>[3x]MEQTEKSKVYAENG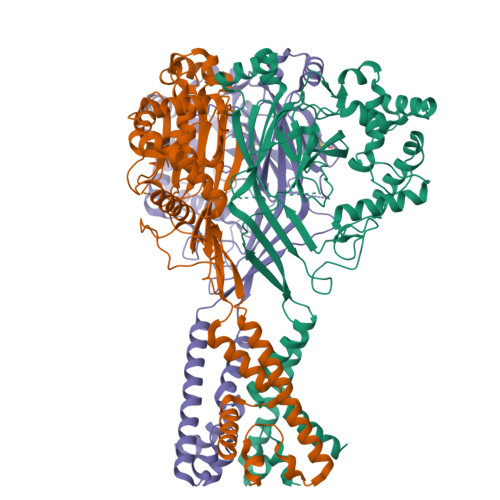LLEKIKLCLSKKPLPSPTERKKFDHDFAISTSFHGIHNIVQNRSKIRRVLWLVVVLGSVSLVTWQIYIRLLNYFTWPTTTSIEVQYVEKMEFPAVTFCNLNRFQTDAVAKFGVIFFLWHIVSKVLHLQEITANSTGSREATDFAASHQNFSIVEFIRNKGFYLNNSTLLDCEFFGKPCSPKDFAHVFTEYGNCFTFNHGETLQAKRKVSVSGRGLSLLFNVNQEAFTDNPALGFVDAGIIFVIHSPKKVPQFDGLGLLSPVGMHARVTIRQVKTVHQEYPWGECNPNIKLQNFSSYSTSGCLKECKAQHIKKQCGCVPFLLPGYGIECDLQKYFSCVSPVLDHIEFKDLCTVGTHNSSCPVSCEEIEYPATISYSSFPSQKALKYLSKKLNQSRKYIRENLVKIEINYSDLNYKITQQQKAVSVSELLADLGGQLGLFCGASLITIIEIIEYLFTNFYWICIFFLLKISEMTQWTPPPQNHLGNKNRIEEC4-(2-THIENYL)-1-(4-METHYLBENZYL)-1H-IMIDAZOLE | 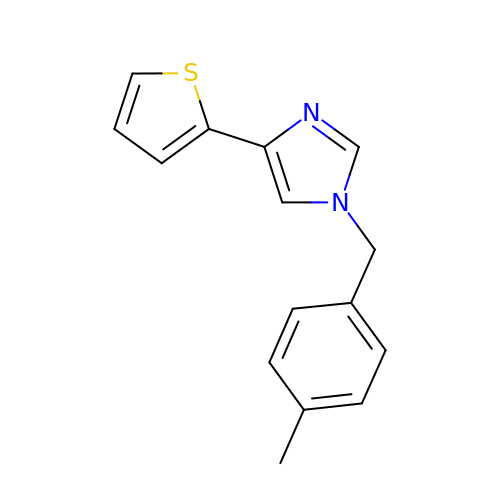C15 H14 N2 S | UMOFOLLUKPBVQG-UHFFFAOYSA-N>QDLDYKDDDDKMSGTKLEDSPPCRDWSSASELDETQEPLLDPTDYDDEEFLRYLWREYLHPKEYAWVLIAGYIIVFVVALIGNVLVCVAVWKNHHM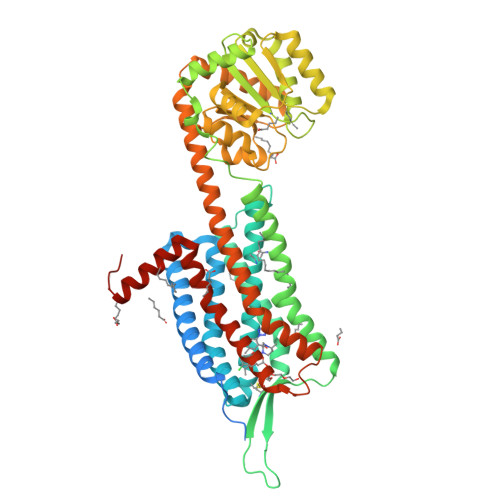RTVTNLFIVNLSLAAVLVTITCLPATLVVDITETWFFGQSLCKVIPYLQTVSVSVSALTLSCIALDRWYAICHPLMFKSTAKRALNSIVIIWIVSCIIMIPQAIVMECSTVFPGLADKTTAFTVCDERWGGEIAPKMYHICFFLVTYAAPLCLMVLLYLQIFRKLWCRQGIDCSFWNESYLTGSRDERKKSLLSKFGMDEGVTFMFIGRFDRGQKGVDVLLKAIEILSSKKEFQEMRFIIIGKGDPELEGWARSLEEKHGNVKVITEMLSREFVRELYGSVDFVIIPSYFEPFGLVALEAMCLGAIPIASAVGGLRDIITNETGILVKAGDPGELANAILKALELSRSDLSKFRENCKKRAMSFSKQIRARRKTARMLMVVVLVFAICYAPISILNVLKRVFGMFAHTEDRETVYAWFAFSHWLVYANSAANPIIYNFLSGKFREEFKAAFSWWWLGVHHHHHHHHHH[2x]> AGHMEKQQRK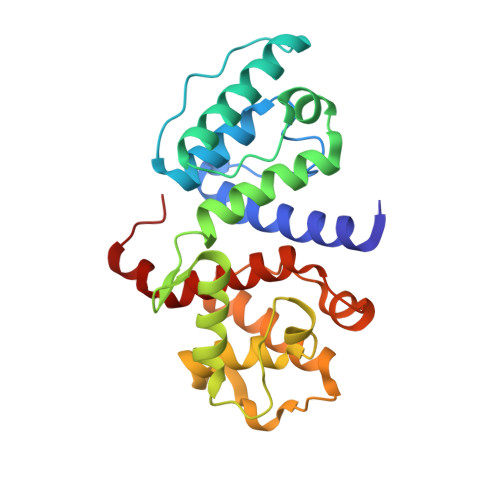TFTAWCNSHLRKAGTQIENIEEDFRDGLKLMLLLEVISGERLAKPERGKMRVHKISNVNKALDFIASKGVKLVSIGAEEIVDGNVKMTLGMIWTIILRFAIQDISVEETSAKEGLLLWCQRKTAPYKNVNIQNFHISWKDGLGFCALIHRHRPELIDYGKLRKDDPLTNLNTAFDVAEKYLDIPKMLDAEDIVGTARPDEKAIMTYVSSFYHAFSGAQEFLEPG>[4x]GSHMS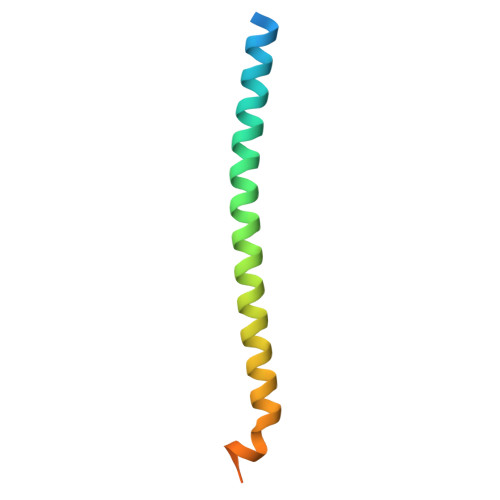NPFDATAGYRSLTYEEVLQELVKHKELLRRKDTHIRELEDYIDNLLVRVMEETPSILRVPYEPSRKAGKFSNS13-BETA-ETHYL-17-ALPHA-ETHYNYL-17-BETA-HYDROXYGON-4-EN-3-ONE | C21 H28 O2 | 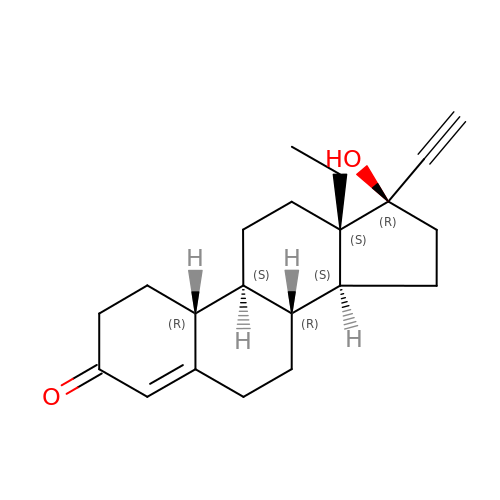WWYNJERNGUHSAO-XUDSTZEESA-N>MSVEGLGKDFCGAIIPDNFFPIEKLRNYTQMGLIRDFAKGSAVIMPGEEITSMIFLVEGKIKLDIIFEDGSEKLLYYAGGNSLIGKLYPTGNNIYATAMEPTRTCWFSEKSLRTVFRTDEDMIFEIFKNYLTKVAYYARQVAEMNTYNPTIRILRLFYELCSSQGKRVGDTYEITMPLSQKSIGEITGVHHVTVSRVLACLKRENILDKKKNKIIVYNLGELKHLSEQ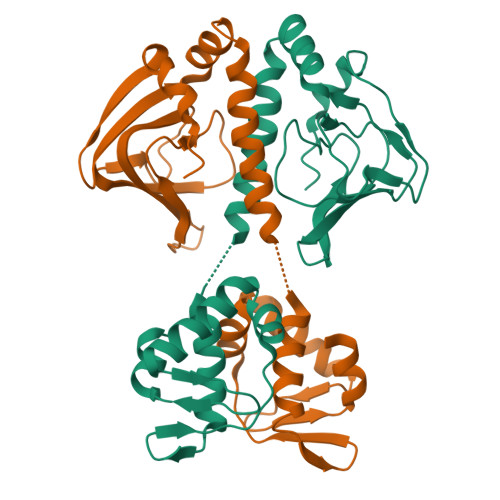TSYYSDPNSSSVDKLAAALDHH[6x]>[2x]GMANFIEKITYLGTPAIKAGNEHLEMI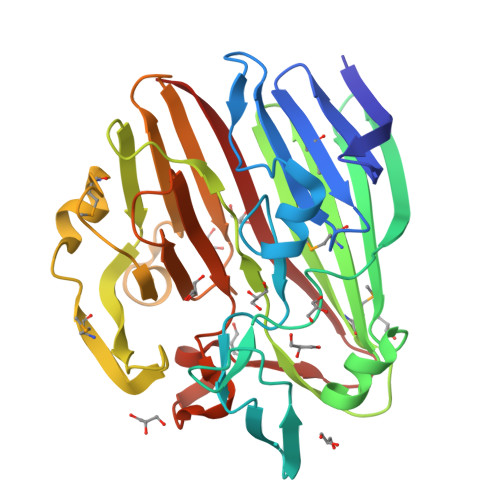VVPEWGSNVISLVDKTTNVQLLREPETAESFHDTPTLYGIPILFPPNRISDGTFSFRGRTYHFDINEKDKHNHLHGFLYHEKWNVVTTKQTDEGVIVETEIDLSELPHVQKQFPHHAVVRMTYTIKENTLFKHATVMNKGKEAFPWGIGYHTTFIFPAESSLFSLTADQQWELDERLLPTGKLMDVPYKEALHEGMDLRHKQLDDVFLSSYQKRGGENQAVIYHQHAHISIIYKADEQFKHWVVYNADGKQGYLCPEPYTWVTNAVNLDLPSSLTGLQVLEPGEETTAKSSITIELNHQ> MNRYALFLVCIFSTSALPAMAALDPSQPLSPAPPLSLFKAWAKPIKPFQITEGVWYVGTKNLSSILLTTPAGHILIDAGLDESAPQIKANIEAAGFRLTDVRYLLNSHARLDQAGGMARLKAWSG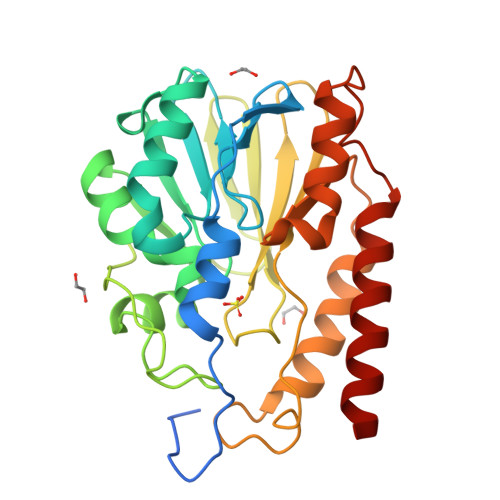AQLVASQPNADQMARGGRQDFALGDALPFPPVTTDKIIHHQESIILGGITVTALFTPGHLPGSTSWRVTLRNGKTLIYADSLATPDYLLINNKNYPDLVTDIQSSFKTLAAQHVDIFIANKGDHFGLLEKRQQLRNGDTQAFFDSNGLQQYVERSRQRFITQLTAQQP> QIVNSVDTMTLTNANVSPDGFTRAGILVNGVHGPLIRGGKNDNFELNVVNDLDNPTMLRPTSIHWHGLFQRGTNWADGADGVNQCPISPGHAFLYKFTPAGHAGTFWYHSHFGTQYCDGLRGPMVIYDDNDPHAALYDEDDENTIITLADWYHIPAPSIQGAAQPDATLINGKGRYVGGPAAELSIVNVEQGKKYRMRLISLSCDPNWQFSIDGHELTIIEVD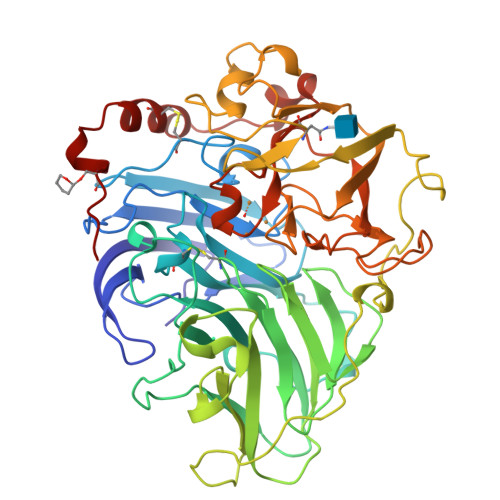GELTEPHTVDRLQIFTGQRYSFVLDANQPVDNYWIRAQPNKGRNGLAGTFANGVNSAILRYAGAANADPTTSANPNPAQLNEADLHALIDPAAPGIPTPGAADVNLRFQLGFSGGRFTINGTAYESPSVPTLLQIMSGAQSANDLLPAGSVYELPRNQVVELVVPAGVLGGPHPFHLHGHAFSVVRSAGSSTYNFVNPVKRDVVSLGVTGDEVTIRFVTDNPGPWFFHCHIEFHLMNGLAIVFAEDMANTVDANNPPVEWAQLCEIYDDLPPEATSIQTVV> SGSTLEMGTCLTNEYDVTGGKAQDFANGRAYWSANTGAFGLVGRINARYSELGGPASWLGYPTSSELKTPDGRGRFVTFEHGSIYWTATTGPWEIPGDMLAAWGTQDYEKGSLGYPTGAAVEYNGGLRQQFEGGYVFRTSNNQSYWVRGEISKKYAEDGIFAQLGFPTGNEKLINGGAFQEFEKGNIYWSASTGAHVILHGDIFDAWGAKGWEQGEYGFPTSDQTAITAGGQTIDFQNGT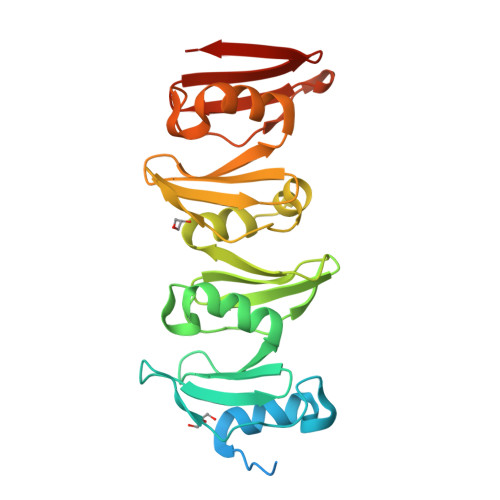IRQVNGRIEESRHHHHHH>[3x]MARTAYNVAFDALKNGKYDDASQLFLSFLELYPN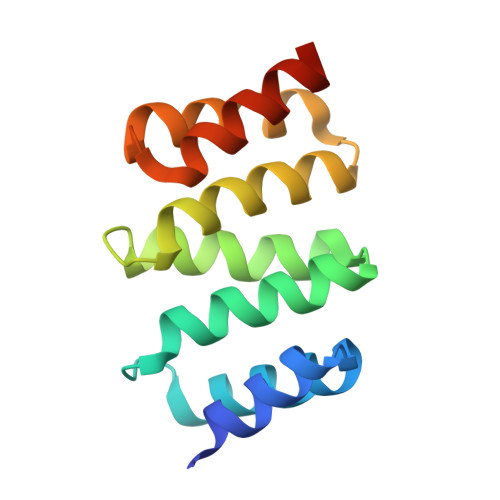GVYTPNALYWLGESYYATRNFQLAEAQFRDLVSRYPTHDKAAGGLLKLGLSQYGEGKNTEAQQTLQQVATQYPGSDAARVAQERLQSIRLGQQLR1-(1,2,3,5,6,7-hexahydro-s-indacen-4-yl)-3-[4-(2-oxidanylpropan-2-yl)furan-2-yl]sulfonyl-urea 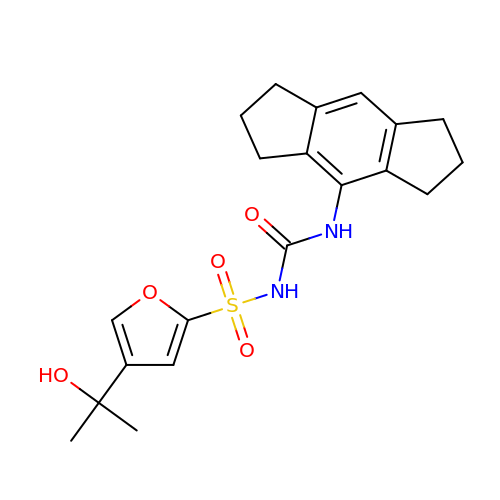| C20 H24 N2 O5 S | HUUSXLKCTQDPGL-UHFFFAOYSA-N3AR,5R,6S,7R,7AR-5-HYDROXYMETHYL-2-METHYL-5,6,7,7A-TETRAHYDRO-3AH-PYRANO[3,2-D]THIAZOLE-6,7-DIOL 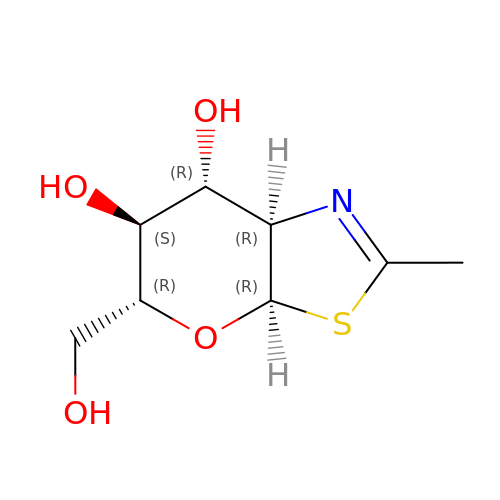| C8 H13 N O4 S | DRHXTSWSUAJOJZ-FMDGEEDCSA-N> AHFEKRFLKRIRDLGEGHFGKVELCRYDPEGDNTGEQVAVKSLKPESGGNHIADLKKEIEILRNLYHENIVKYKGICTEDGGNGIKLIMEFLPSGSLKEYLPKNKNKINLKQQLKYAVQICKGMDYLGSRQYVHRDLAARNVLVESEHQVKIGDFGLTKAIETDKEYYTVKDDRDSPVFWYAPECLMQSKFYIASDVWSFGVTLHELLTYCDSDSSPMALFLKMIGPTHGQMTVTRLVNTLKEGKRLPCPPNCPDEV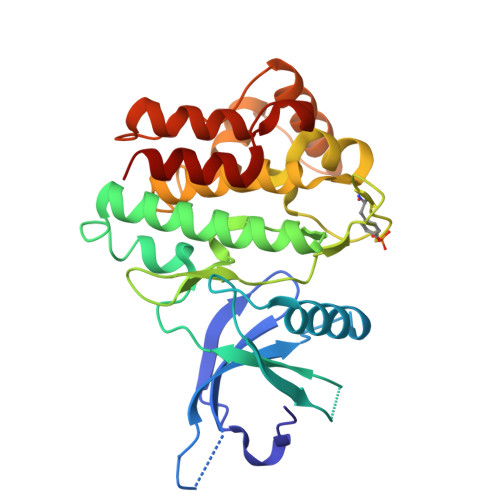YQLMRKCWEFQPSNRTSFQNLIEGFEALL> YALXRQ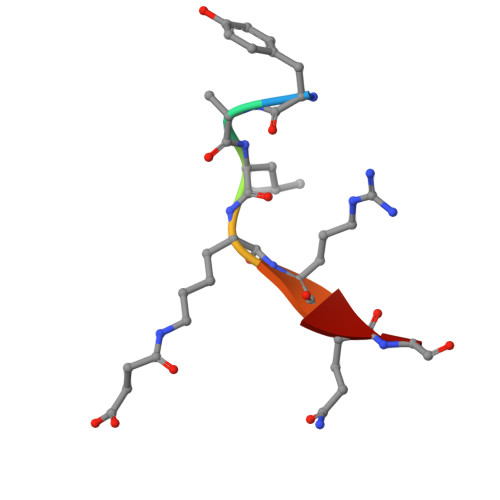G>[2x]ADTMTFTAKNGNVTFDHKKHQTIVPDCAVCHGKTPGKIEGFGKEM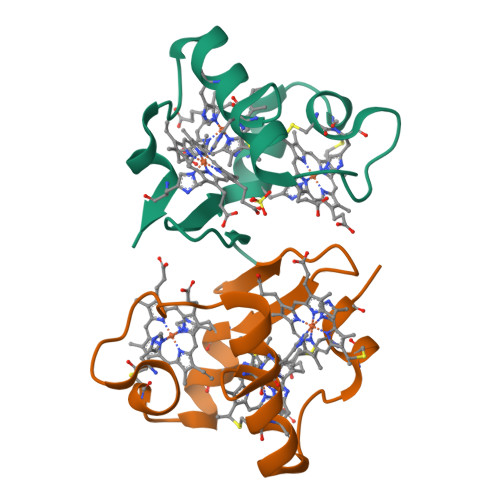AHGKSCKGCHEEMKKGPTKCGECHKK>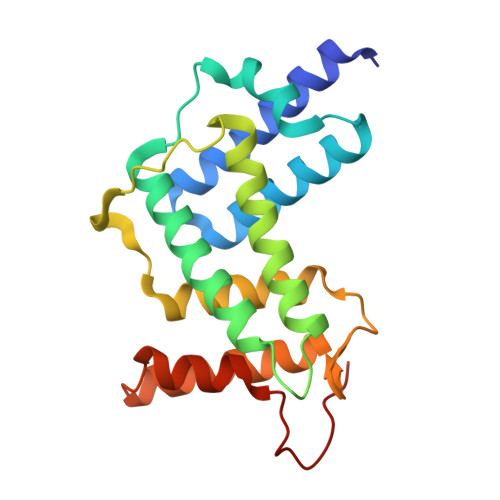 GHMVTRIENLENAKKLWDNANSMLEKGNISGYLKAANELHKFMKEKNLKEDDLRPELSDKTISPKGYAILQSLWGAASDYSRAAATLTESTVEPGLVSAVNKMSAFFMDCKLSPNERATPDPDFKVGKSKILVGIMQFIKDVADPTSKIWMHNTKALMNHKIAAIQKLERSNNVNDETLESVLSSKGENLSEYLSYK> MQYDDDWQYEDCKLARDGPPATIVAIDEESRNGTILVDNMLIKGTAGGPDPTIELSLKDNVDYWVLMDPVKQMLFLNSTGRVLDRDPPMNIHSIVVQVQCINKKVGTIIYHEVRIVVRDRNDNSPTFKHESYYATVNELTPVGTTIFTGFSGDNGATDIDDGPNGQIEYVIQYNPDDPTSNDTFEIPLMLTGNIVLRKRLNYEDKTR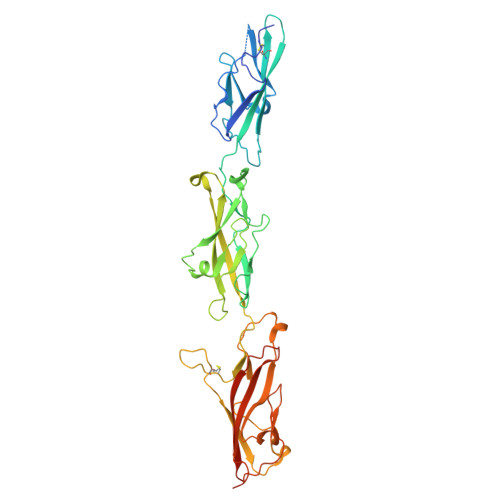YFVIIQANDRAQNLNERRTTTTTLTVDVLDGDDLGPMFLPCVLVPNTRDCRPLTYQAAIPELRTPEELNPIIVTPPIQAIDQDRNIQPPSDRPGILYSILVGTPEDYPRFFHMHPRTAELSLLEPVNRDFHQKFDLVIKAEQDNGHPLPAFAGLHIEILDENDNLEHHHHHH2-fluoranyl-3-[6-[1-(4-fluoranyl-3-oxidanyl-phenyl)ethenyl]pyridin-2-yl]phenol 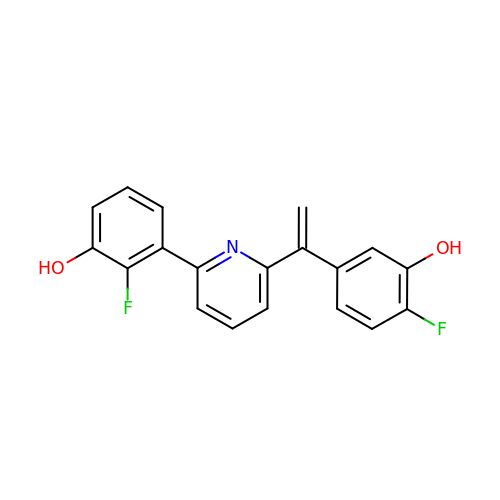| C19 H13 F2 N O2 | LSHVGZUGKOCADJ-UHFFFAOYSA-N Our work utilizes biotin–streptavidin (Sav) technology to develop artificial metalloproteins (ArMs) that mimic the active sites of natural copper metalloenzymes. Our group develops artificial metalloproteins (ArMs) using biotin–streptavidin (Sav) technology to mimic natural metalloenzyme active sites to characterize otherwise elusive intermediates and study the effects of the secondary coordination sphere on metal ion(s) reactivity. This approach leverages the strong binding affinity between biotinylated metal complexes and the Sav host to confine synthetic metal cofactors within a protein scaffold. By engineering ArMs with aromatic residues within their secondary coordination spheres, we systematically investigate the influence of these residues on Cu reactivity and oxidant activation. Our results demonstrate how the inclusion of aromatic residues within the secondary coordination sphere influences the structure and reactivity of copper ArMs.

Notice that the relative abundance of the m/z peak consistent with the singly oxidized species increases and replaces that of the unoxidized species as the most abundant. These results contrast with those obtained with 2, where in the absence of tyrosine, only a small amount of oxidation occurs (new peak at 16 381.2 m/z) and the unoxidized peak (16 364.8 m/z) remains the most abundant. Upon reaction of 2 with H2O2, we could identify the triply charged DF31 ([DF313+], 1055.5 m/z, retention time 3.1 min), and a relatively small amount of the singly and doubly oxidized species, though their relative abundance is significantly less than in 1. The premise that S112Y is modified due to its positioning was supported by LC-MS (and MS/MS) analysis of the trypsin digestion of 2 and 3, where treatment with H2O2 resulted in only minor modification of the DF31 peptide (G and S20†).

> MASMTGGQQMGRDEAGITGTWYNQLGSTFIVTAGADGALTGTYESAVGNAESRYVLTGRYDSAPATDGSGTALGWTVAWKNNYRNAHSATTWSGQYVGGAQARINTQWLLTSGTTEANAWASTLVGHDTFTKVKPSAASIDAAKKAGVNNGNPLDAVQQ> GKTKEGV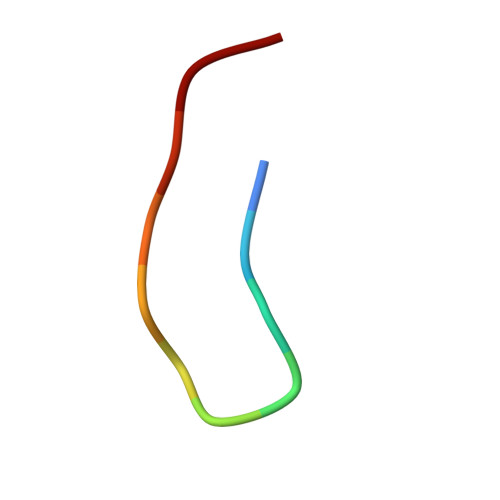LYVG> MKIVKPQPFTFKGGKKAVLLLHGFTGNTA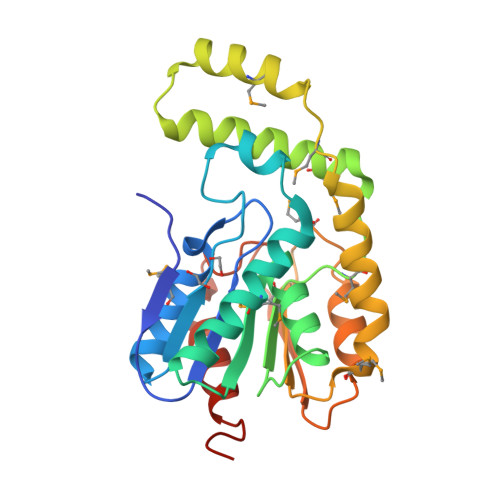DVRMLGRYLNEKGYTCHAPQYKGHGVPPEELLSTGPEDWWKDVMDGYEYLKSEGYEQIAACGLSLGGVFSLKLGYTVPIKGIVPMCAPMYIKSEETMYEGVLDYARNYKKFEGKTAEQINAEMEEFKKTPMNTLKALQDLIADVREHVDMIYSPTFVVQARHDHMINTDSANIIYNEVETDDKQLKWYEESGHAITLDKERETLHKDVYQFLETLDWQTHHHHHH> MGKSAVIFVERATPATLTELKDALSNSILSVRDPWSIDFRTYRCSIKNLPADVSKLMYSITFHHHGRQTVLIKDNSAMVTTAAAADIPPALVFNGSSTGVPESIDTILSSKLSNIWMQRQLIKGDAGETLILDGLTVRLVNLFS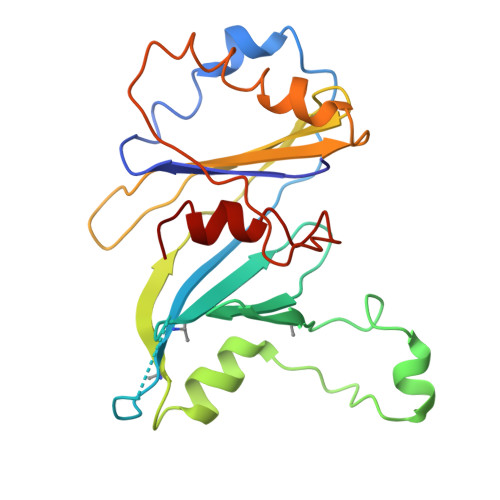STGFKGLLIELQADEAGEFETKIAGIEGHLAEIRAKEYKTSSDSLGPDTSNEICDLAYQYVRALEL> MKITNDTTTYEVAELMGSEADELD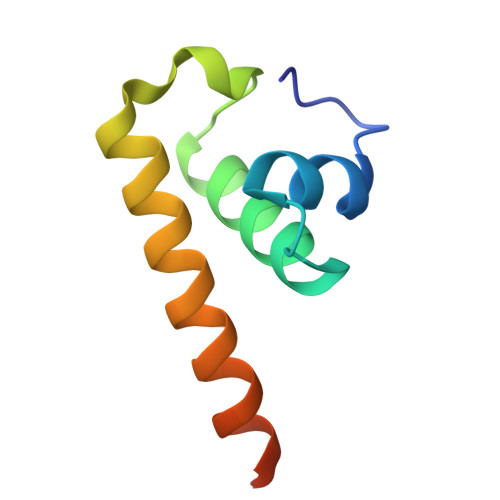GRIMMGLLSRECVVDTDDLSEDQWLALIDESQKVRREQFESDEALEHHHHHH>MGSSHHHHHHSQDLASAEAGITGTWYNQSGSTFTVTAGADGNLTGQYENRAQGTGCQNSPYTLTGRYNGTKLEWRVEWNNSTENCHSRTEWRGQYQGGAEARINTQWNLTYEGGSGPATEQGQDTFTKVKPSAASGSDYKDDDDK[6x]

Tetrameric streptavidin (T-Sav) has been popularly used, engineered and evolved for hosting reactions that are mediated by biotin-appended chemical catalysts. We have recently reported an organocatalytic 1,4 conjugate addition of nitromethane to cinnamaldehydes within a protein environment through adaptation of the streptavidin–biotin technology. In this system, biotin was covalently modified with pyrrolidine groups, resulting in ligands 1 and 2 which differ by one stereocenter. Here, we performed mechanistic investigations on how a protein host affects iminium catalysis.

The monomeric variant M-Sav was tested as an alternative host for iminium catalysis. Although it lacks the subunit interface and shares moderate sequence identity with T-Sav (55%), M-Sav has high affinity to biotin (KD = 2.8 nM). Catalysis by 2 in M-Sav was mildly improved (20% 1,4-addition product, entry 2) but there remained a substantial amount of the 1,2-addition side product (7%). The melting temperature of M-Sav increased significantly when ligand 1 or 2 was included (+20 °C) as assessed by circular dichroism spectroscopy (Fig. S2†), implying its binding to the biotinylated catalysts. We began by testing the monomeric M-Sav as the host; the reaction lacks both enantio- and regioselectivity despite numerous optimization attempts, and protein X-ray crystallography analysis revealed that the catalyst is solvent exposed. Tyr111 in M-Sav : 2 is a relatively bulky residue located in proximity to the secondary amine motif and corresponds to Ser112 in T-Sav : 2. Replacing Tyr111 with other residues including serine, threonine, valine, lysine and alanine did not improve the conversion or the regioselectivity (entries 3–7). Glu120 in M-Sav : 2 is in proximity and spatially corresponds to Leu124 in T-Sav : 2. Though modifying Glu120 slightly improved the overall yield of the 1,4-addition product, the enantioselectivity of the catalysis remained low (entry 8). In contrast, the monomeric M-Sav contains a solvent-exposed site and was found to be a poor host for iminium catalysis.> MSLPGTGSGTSSGGGNTQGQDVYII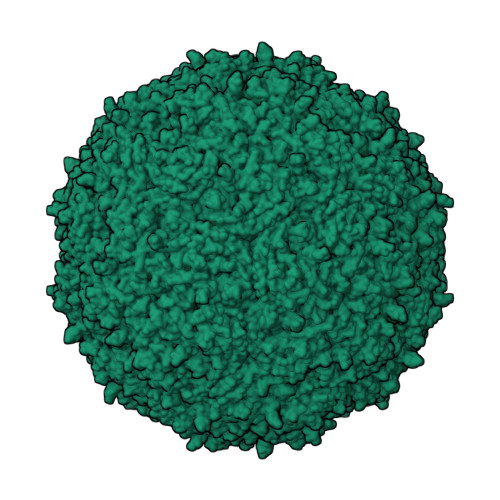PRPFSNFGKKLSTYTKSHKFMIFGLANNVIGPTGTGTTAVNRLLTTCLAEIPWQKLPLYMNQSEFDLLPPGSRVVECNVKVIFRTNRIAFETSSTVTKQATLNQISNVQTAIGLNKLGWGINRAFTAFQSDQPMIPTATTAPKYEPVTGDTGYRGMIADYYGADSTNDTAFGNAGNYPHHQVSSFTFLQNYYCMYQQTNQGTGGWPCLAEHLQQFDSKTVNNQCLIDVTYKPKMGLIKSPLNYKIIGQPTVKGTISVGDNLVNMRGAVVTNPPEATQNVAESTHNLTRNFPADLFNIYSDIEKSQVLHKGPWGHENPQIQPSVHIGIQAVPALTTGALLINSSPLNSWTDSMGYIDVMSSCTVMEAQPTHFPFSTEANTNPGNTIYRINLTPNSLTSAFNGLYGNGATLGNV>MGHHHHHHHHEFIPSNTDYPGPHHFEVTFQQSST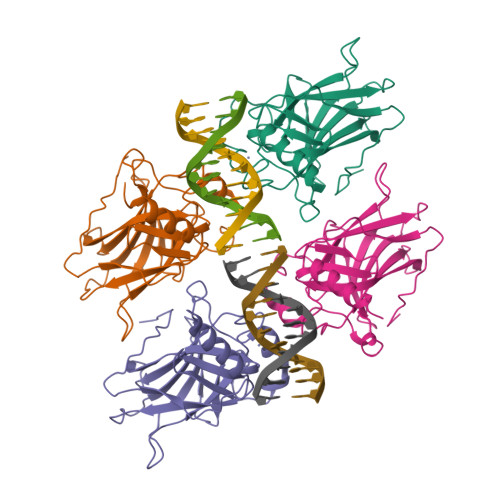AKSATWTYSPLLKKLYCQIAKTCPIQIKVSTPPPPGTAIRAMPVYKKAEHVTDVVKRCPNHELGRDFNEGQSAPASHLIRVEGNNLSQYVDDPVTGRQSVVVPYEPPQVGTEFTTILYNFMCNSSCVGGMNRRPILIIITLEMRDGQVLGRRSFEGRICACPGRDRKADEDHYREQ[8x]> MENFRKVRSEEAPAGCGAEGGGPGSGPFADLAPGAVHMRVKEGSKIRNLMAFATASMAQPATRAIVFSGCGRATTKTVTCAEILKRRLAGLHQVTRLRYRSVREVWQSLPPGPTQGQTPGEPAASLSVLKNVPGLAILLSKDALDPRQPGYQPPNPHPGPSSPPAA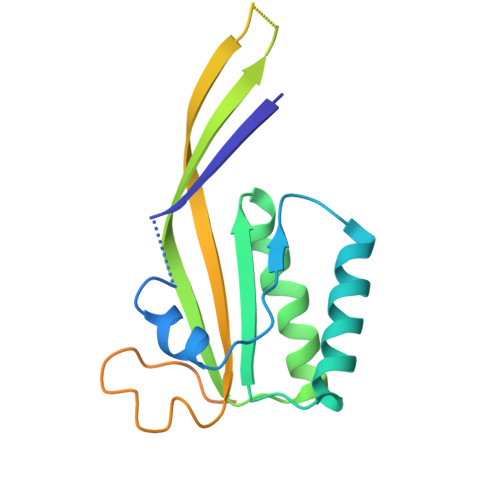PASKRSLGEPAAGEGSAKRSQPEPGVADEDQTA4-[(4-{[4-(4-cyano-2,6-dimethylphenoxy)thieno[3,2-d]pyrimidin-2-yl]amino}piperidin-1-yl)methyl]benzene-1-sulfonamide 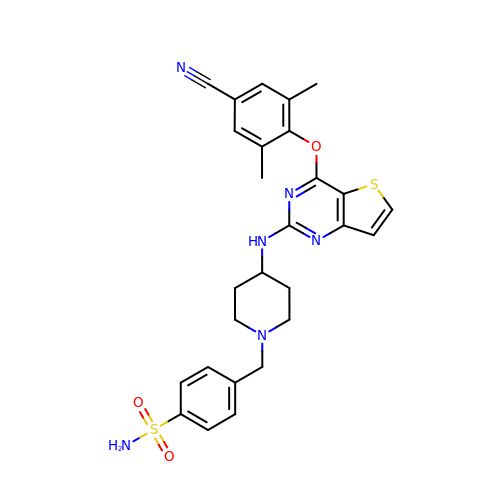| C27 H28 N6 O3 S2 | ZTRXHQCTETXYCC-UHFFFAOYSA-N One such TUT family member, Cid1 from Schizosaccharomyces pombe, is a now well-characterized TUT, which was first demonstrated to be localized to the cytoplasm and to possess poly(A) polymerase activity in vitro, but more recently has been shown to possess TUT or poly(U) polymerase activity, in vitro and in vivo. The TUTactivity of Cid1 has been shown to be important in promoting mRNA degradation of polyadenylated and 3′ trimmed transcripts mediated by Lsm1–7 and the exonuclease Dis3l2 (12,13). Cid1 has been extensively characterized both structurally and biochemically, revealing that a single histidine (H336) in the nucleotide recognition motif (NRM) is predominantly responsible for discriminating uracil over other bases via a mechanism that was proposed to involve two alternative conformations of the H336 side chain. We used an RNA-binding-defective mutant of Cid1 (K133A/R137A/R277A/K282A) to improve the resolution of our crystal diffraction for higher resolution studies.

A β-trapdoor structure (residues 310–322) was previously observed bridging the N- and C-terminal domains of Cid1 in a UTP-bound crystal structure and was suggested to play a role in UTP selectivity and enzyme function via substrate containment as part of an induced-fit mechanism. Deployment of the trap door correlated with H336 side chain flipping but its absence from the Apo crystal form and other UTP-bound forms suggested that its stabilization depends on direct contact with the CTD. In addition to the novel structure (crystal form I, space group P1) described in detail above we were able to crystallize the RNA-binding mutant of Cid1 in yet another crystal form (crystal form II, space group P21), which is also an Apo state but this time with an observable β-trapdoor. However in this case the β-trapdoor does not bridge the two domains but instead is stabilized by contacting a crystallographically-related molecule. Normal mode analysis of the model, complete with its β-trap door, demonstrates that this feature is comparatively more flexible than the majority of the CTD. This strongly suggests that the ordering of the trap door which we have observed previously is fundamentally a property of interaction with the NTD and not of NTP binding itself, because it can be mimicked by a crystal contact. We suggest that this enables the trap door to act as a ‘strut’ preventing the collapse of the catalytic cleft when enzyme substrates are bound but before uridylylation has occurred.

>SHKEFTKFCYEVYNEIKISDKEFKEKRAALDTLRLCLKRISPDAELVAFGSLESGLALKNSDMDLCVLMDSRVQSDTIALQFYEELIAEGFEGAFLQAARIPIIKLTSDTKNGFGASFQCDIGFNNRLAIHNTLLLSSYTKLDARLKPMVLLVKHWAKRKQINSPYFGTLSSYGYVLMVLYYLIHVIKPPVFPNLLLSPLKQEKIVDGFDVGFDDKLEDIPPSQNYSSLGSLLHGFFAFYAYAFEPREKVVTFRRPDGYLTKQEKGWTSATEHTGSADQIIKDRYILAIEDPFEISHNVGRTVSSSGLYRIRGEFMAASRLLNSRSYPIPYDSLFEEAPIPPRRQKKTDEQSNKKLLNETDGDNSE[2x]>GMISYLKKAEKTPQTETATAQKVVTEMLAEIQARGKDAVRQYAKQLDGWSGDIVLTPDQIREQTKDVPAGVRADIDFAIRQVTDFALAQRESLKEFSVELHPGVTAGQRVLPVNVVGCYAPAGRYAHIASAYMGVATAKAAGVKTVVACSSPFRGQGIHPHVLYAFQAAGADVIMALGGVQAIASMAYGLFTGKPADVVVGPGNKFVAEAKRSLYGQVGIDVFAGPSEVAVIADETADPAIVASDLVGQAEHGHESPAWLFTTSRDLADRVMALVPELIAKLPPTARDAATAAWRDYGEVILCGTREEVVEISDRYASEHLEVHTADLDWWLANLTCYGSLFLGEETTVAFGAKTSGPNHVLPTKGAARYSGGLSVHKFMKTLTWQQMTREATRQIGQVTARISRLEGMEAHARTADDRMAKYFPNASFEMGTPVEV[2x]

Here, we study DHPS-3-dehydrogenase from Cupriavidus pinatubonensis (CpHpsN), a bacterium capable of utilizing DHPS as a sole carbon source. Kinetic analysis of CpHpsN reveals a strict preference for R-DHPS, catalyzing its 4-electron oxidation to R-SL, with high specificity for NAD+ over NADP+. CpHpsN forms a domain-swapped tight dimer with 28% of surface area buried at the dimer interface, with the interface featuring extensive hydrophobic and hydrogen-bond interactions. Domain 4 lies at the C-terminus and contributes to the active site and is also involved in dimerization through a metal binding site. Coordination of Zn2+ involves three residues from one monomer and one residue (His411*; * denotes the other monomer in the dimer) from the other monomer (Fig. 5 and S7†), showing that the enzyme forms an obligate dimer.

To probe the roles of Glu318, His319 and Asp352, we conducted site-directed mutagenesis to convert each residue independently to Ala. No activity was detected for the D352A mutant of CpHpsN, most likely due to the inability to form a productive zinc-coordination complex with substrate. The 3D structure of the CpHpsN D352A mutant in complex with Zn2+ and NAD+ was solved and refined to 2.23 Å resolution and is essentially identical to the CpHpsN·Zn2+·NADH structure in the ‘open’ conformation (Fig. S12a–c†). Collectively, these data provide evidence for a role for Asp352 in zinc coordination to form a catalytically productive complex, and for Glu318 and His319 in the catalytic mechanism of CpHpsN.> EMAESVSRPQRPPVIWIGAQECTGCTESLLRATHPTVENLVLETISLEYHEVLSAAFGHQVEENKHNALEKYKGQYVLVVDGSIPLKDNGIYCMVAGEPIVDHIRRAAEGAAAIIAIGSCAAWGGVAAAGVNPTGAVGLQEVLPGKTIINIPGCPPNPHNFLATVAHIITYGKPPKLDAKNRPTFAYGRLIHEHCERRPHFDAGRFAKEFGDEGHREGWCLYHLGCKGPETYGNCSTLQFCDVGGVWPVAIGHPCYGCNEEGIGFHKGIHQLAHVENQTPRSEKPD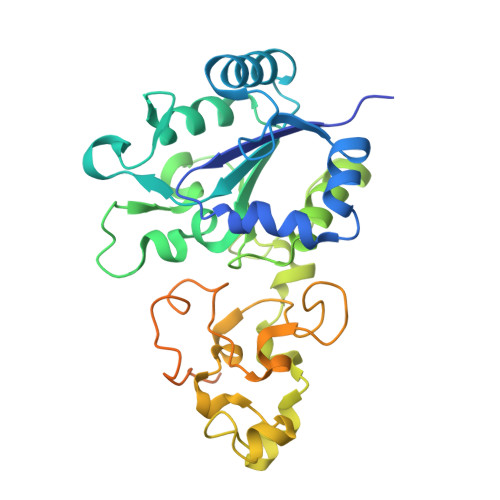VNIKEGGNISAGAVGLLGGVVGLVAGVSVMAVRELGRQQKKDNADSRGE> NLFVALY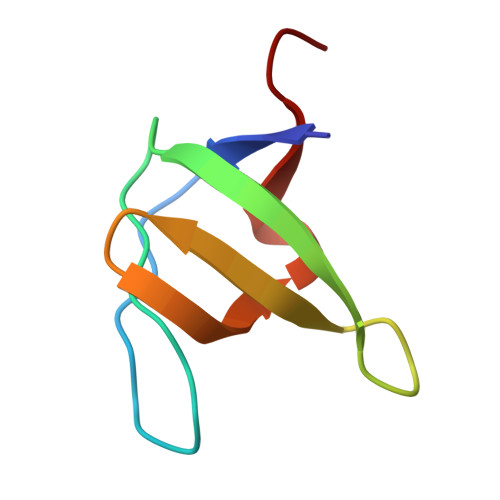DFVASGDNTLSITKGEKLRVLGYNHNGEWCEAQTKNGQGWVPSNYITPVNS> STLRLLISDSYDPWFNLA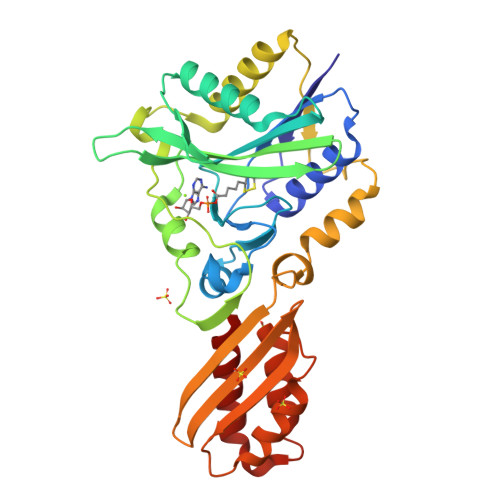VEECIFRQMPATQRVLFLWRNADTVVIGRAQNPWKECNTRRMEEDNVRLARRSSGGGAVFHDLGNTCFTFMAGKPEYDKTISTSIVLNALNALGVSAEASGRNDLVVKTVEGDRKVSGSAYRETKDRGFHHGTLLLNADLSRLANYLNPDKKKLAAKGITSVRSRVTNLTELLPGITHEQVCEAITEAFFAHYGERVEAEIISPNKTPDLPNFAETFARQSSWEWNFGQAPAFSHLLDERFTWGGVELHFDVEKGHITRAQVFTDSLNPAPLEALAGRLQGCLYRADMLQQECEALLVDFPEQEKELRELSAWMAGAVR> ADQRRDFIDIESKFALRTPEDTAEDTCHLIPGVAESVATCHFNHSSKTFMVIHGWTVTGMYESWVPKLVAALYKREPDSNVIVVDWLSRAQEHYPVSAGYTKLVGQDVARFINWMEEEFNYPLDNVHLLGYSLGAHAAGIAGSLTNKKVNRITGLDPAGPNFEYAEAPSRLSPDDADFVDVLHTFTRGSPGRSIGIQKPVGHVDIYPNGGTFQPGCNIGEAIRVIAER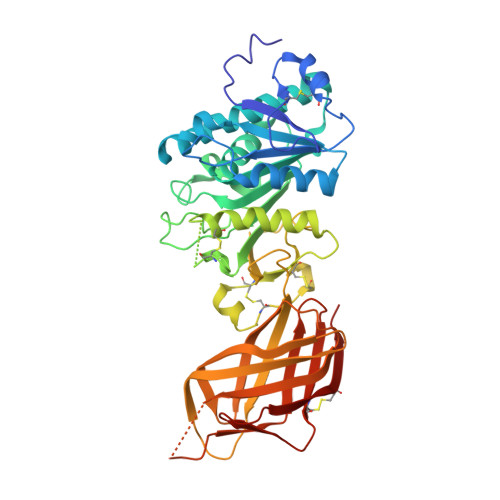GLGDVDQLVKCSHERSIHLFIDSLLNEENPSKAYRCSSKEAFEKGLCLSCRKNRCNNLGYEINKVRAKRSSKMYLKTRSQMPYKVFHYQVKIHFSGTESETHTNQAFEISLYGTVAESENIPFTLPEVSTNKTYSFLIYTEVDIGELLMLKLKWKSDSYFSWSDWWSSPGFAIQKIRVKAGETQKKVIFCSREKVSHLQKGKAPAVFVKCHDKSLNKKSG> MAAFVSGGCGVGGQRRAWPAKGAAVARTHACPTTMVVLPVARAGLAATAKKNQYMGTSVAPEIVLTDKGSDMSRKVKTEDKK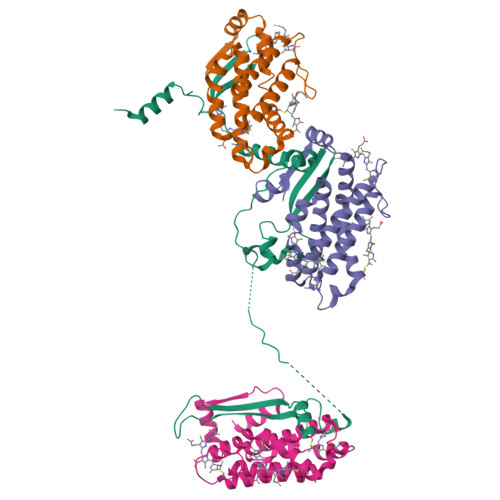VAADQAAAMGILANMSLYASLNPVKRMTYKAKEQAPAYVKKTGNPVEDFYPSSWRNMAPVISLSANRVAVAFEKIDAASNGVKANSNNKPFWKSGATTKNYVAPEAPAQSEPETLDDAAYQRYFPARIRNKAPAMEFRRPSFANTEDPSAYFMLQKETVPLRMALAEKLLTKLGRKGDGSEAEEEKVKPQKKAAKKDAKDDAKDDE;>[3x]MLDAFSRVVVNSDAKAAYVGGSDLQALKSFIADGNKRLDAVNSIVSNASCMVSDAVSGMICENPGLISPGGNCYTNRRMAACLRDGEIILRYVSYALLAGDASVLEDRCLNGLKETYIALGVPTNSSIRAVSIMKAQAVAFITNTATERKMSFAAGDCTSLASEVASYFDRVGAAIS>SAAATQAVPAPNQQPEVFCNQIFINNEWHDAVSRKTFPTVNPSTGEVICQVAEGDKEDVDKAVKAARAAFQLGSPWRRMDASHRGRLLNRLADLIERDRTYLAALETLDNGKPYVISYLVDLDMVLKCLRYYAGWADKYHGKTIPIDGDFFSYTRHEPVGVCGQIIPWNFPLLMQAWKLGPALATGNVVVMKVAEQTPLTALYVANLIKEAGFPPGVVNIVPGFGPTAGAAIASHEDVDKVAFTGSTEIGRVIQVAAGSSNLKRVTLELGGKSPNIIMSDADMDWAVEQAHFALFFNQGQCSCAGSRTFVQEDIYDEFVERSVARAKSRVVGNPFDSKTEQGPQVDETQFKKILGYINTGKQEGAKLL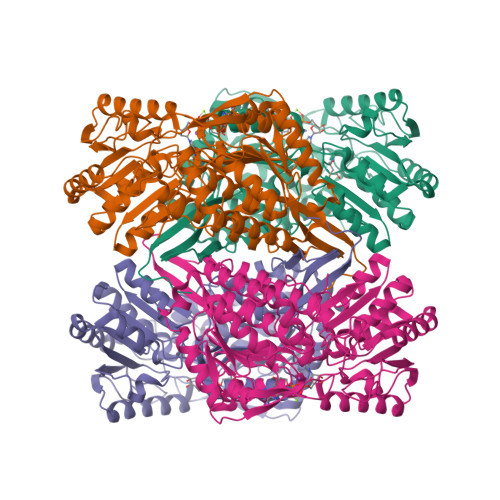CGGGIAADRGYFIQPTVFGDVQDGMTIAKEEIFGPVMQILKFKTIEEVVGRANNSTYGLAAAVFTKDLDKANYLSQALQAGTVWVNCYDVFGAQSPFGGYKMSGSGRELGEYGLQAYTEVKTVTVKVPQKNS[8x]> MREEFLEEIPLDAPPEEAKELRTEVMTLNVGPQHPSTHGVLRLMVTLSGEEVLEVVPHIGYLHTGFEKTMEHRTYLQNITYTPRMDYLHSFAHDLAYALAVEKLLGAVVPPRAETIRVILNELSRLASHLVFLGTGLLDLGALTPFFYAFRERETILDLFEWV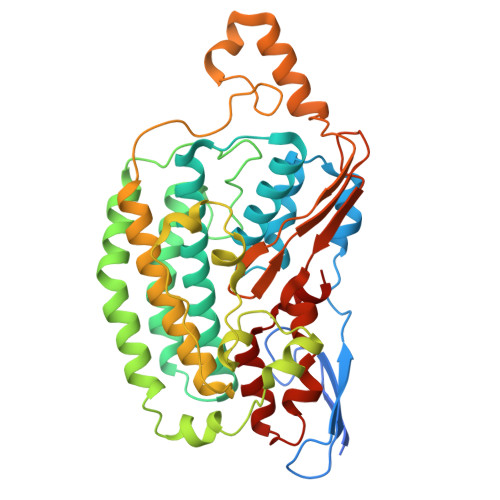TGQRFHHNYIRIGGVKEDLPEEFVPELKKLLEVLPHRIDEYEALFAESPIFYERARGVGVIPPEVAIDLGLTGGSLRASGVNYDVRKAYPYSGYETYTFDVPLGERGDVFDRMLVRIREMRESVKIIKQALERLEPGPVRDPNPQITPPPRHLLETSMEAVIYHFKHYTEGFHPPKGEVYVPTESARGELGYYIVSDGGSMPYRVKVRAPSFVNLQSLPYACKGEQVPDMVAIIASLDPVMGDVDR>MSSLLVKKLVESATTPMRGSEGAAGYDISSVEDVVVPAMGRIAVSTGISIRVPDGTY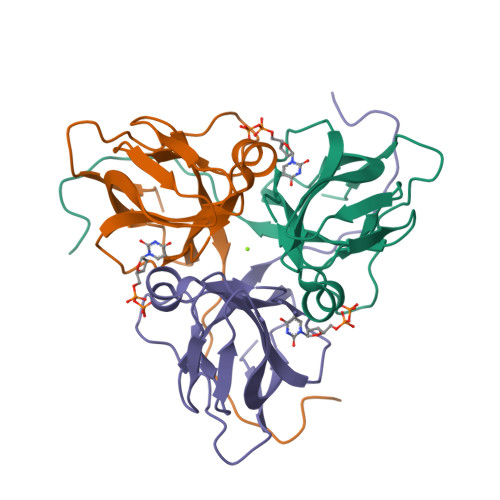GRIAPRSGLAYKYGIDVLAGVIDSDYRGEVKVILYNTTERDYIIKKGDRIAQLILEQIVTPGVAVVLDLSDTARGSGGFGSTGI[4x]> MSAALPSIQLPVDYNNLFNEITDFLVTFKQDTLSSDATRNENEDENLDAENIEQHLLEKGPKYMAMLQKVANRELNSVIIDLDDILQYQNEKFLQGTQADDLVSAIQQNANHFTELFCRAIDNNMPLPTKEIDYKDDVLDVILNQRRLRNERMLSDRTNEIRSENLMDTTMDPPSSMNDALREVVEDETELFPPNLTRRYFLYFKPLSQNCARRYRKKAISSKPLSVRQIKGDFLGQLITVRGIITRVSDVKPAVEVIAYTCDQCGYEVFQEVNSRTFTPLSECTSEECSQNQTKGQLFMSTRASKFSAFQECKIQELSQQVPVGHIPRSLNIHVNGTLVRSLSPGDIVDVTGIFLPAPYTGFKALKAGLLTETYLEAQFVRQHKKKFASFSLTSDVEERVMELITSGDVYNRLAKSIAPEIYGNLDVKKALLLLLVGGVDKRVGDGMKIRGDINVCLMGDPGVAKSQLL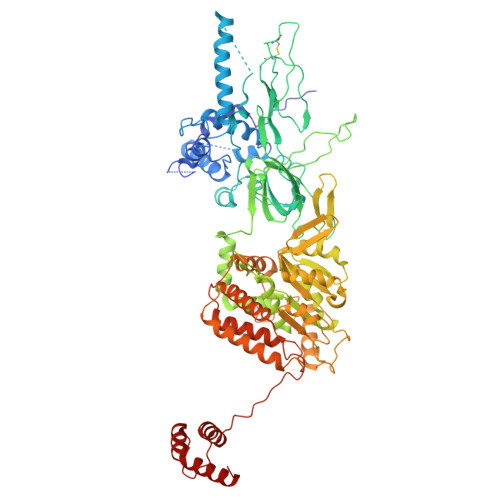KAICKISPRGVYTTGKGSSGVGLTAAVMKDPVTDEMILEGGALVLADNGICCIDEFDKMDESDRTAIHEVMEQQTISISKAGINTTLNARTSILAAANPLYGRYNPRLSPLDNINLPAALLSRFDILFLMLDIPSRDDDEKLAEHVTYVHMHNKQPDLDFTPVEPSKMREYIAYAKTKRPVMSEAVNDYVVQAYIRLRQDSKREMDSKFSFGQATPRTLLGIIRLSQALAKLRLADMVDIDDVEEALRLVRVSKESLYQETNKSKEDESPTTKIFTIIKKMLQETGKNTLSYENIVKTVRLRGFTMLQLSNCIQEYSYLNVWHLINEGNT> EDPEVLFKNKGCVACHAIDTKKVGPAYADVAKKYAGRKDAVDYLAGKIKKGGSGVWGSVPAPPQNVTD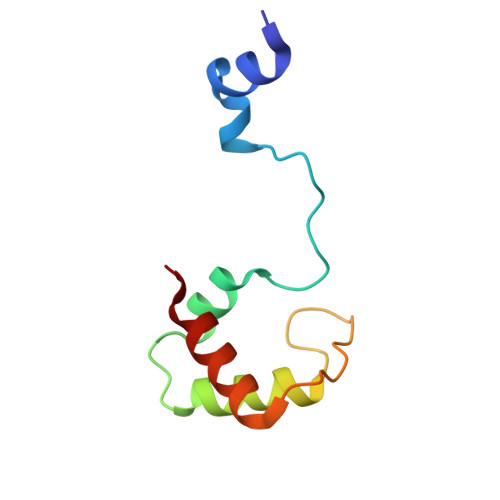AEAKQLAQWILSIK> GGSKMEYEWKPDEQGLQQILQLLKESQSPDTTIQRTVQQKLEQLNQYPDFNNYLIFVLTKLKSEDEPTRSLSGLILKNNVKAHFQNFPNGVTDFIKSECLNNIGDSSPLIRATVGILITTIASKGELQNWPDLLPKLCSLLDSEDYNTCEGAFGALQKICEDSAEILDSDVLDRPLNIMIPKFLQFFKHSSPKIRSHAVACVNQFIISRTQALMLHIDSFIENLFALAGDEEPEVRKNVCRALVMLLEVRMDRLLPHMHNIVEYMLQRTQDQDENVALEACEFWLTLAEQPICKDVLVRHLPKLIPVLVNGMKYS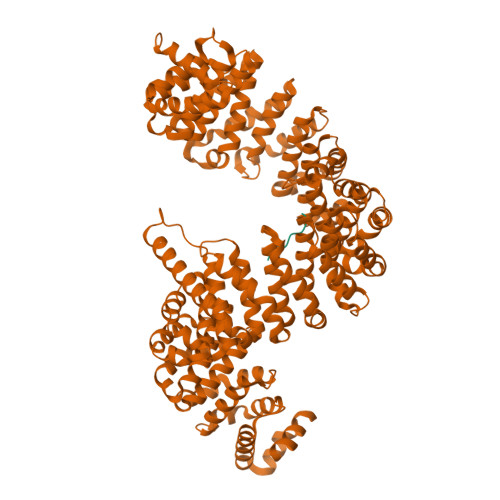DIDIILLKGDVEEDETIPDSEQDIRGGSGGSGDTISDWNLRKCSAAALDVLANVYRDELLPHILPLLKELLFHHEWVVKESGILVLGAIAEGCMQGMIPYLPELIPHLIQCLSDKKALVRSITCWTLSRYAHWVVSQPPDTYLKPLMTELLKRILDSNKRVQEAACSAFATLEEEACTELVPYLAYILDTLVFAFSKYQHKNLLILYDAIGTLADSVGHHLNKPEYIQMLMPPLIQKWNMLKDEDKDLFPLLECLSSVATALQSGFLPYCEPVYQRCVNLVQKTLAQAMLNNAQPDQYEAPDKDFMIVALDLLSGLAEGLGGNIEQLVARSNILTLMYQCMQDKMPEVRQSSFALLGDLTKACFQHVKPCIADFMPILGTNLNPEFISVCNNATWAIGEISIQMGIEMQPYIPMVLHQLVEIINRPNTPKTLLENTAITIGRLGYVCPQEVAPMLQQFIRPWCTSLRNIRDNEEKDSAFRGICTMISVNPSGVIQDFIFFCDAVASWINPKDDLRDMFCKILHGFKNQVGDENWRRFSDQFPLPLKERLAAFYGV;> IGRLHKQRKPDRRKRSRPY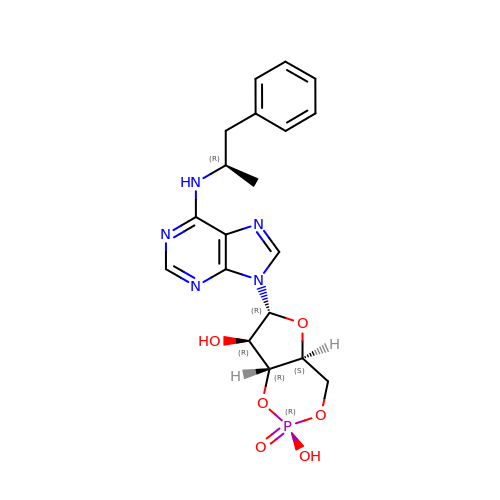(2R)-N6-(1-Methyl-2-phenylethyl)adenosine-3',5'-cyclic monophosphate | C19 H22 N5 O6 P | MKYZONTUKKUGCB-OCXLHJLWSA-N> GPHMATGQDRVVALVDMDCFFVQVEQRQNPHLRNKPCAVVQYKSWKGGGIIAVSYEARAFGVTRSMWADDAKKLCPDLLLAQVRESRGKANLTKYREASVEVMEIMSRFAVIERASIDEAYVDLTSAVQERLQKLQGQPISADLLPSTYIEGLPQGPTTAEETVQKEGMRKQGLFQWLDSLQIDNLTSPDLQLTVGAVIVEEMRAAIERETGFQCSAGISHNKVLAKLACGLNKPNRQTLVSHGSVPQLFSQMPIRKIRSLGGKLGASVIEILGIEYMGELTQFTESQLQSHFGEKNGSWLYAMCRGIEHDPVKPRQLPKTIGCSKNFPGKTALATREQVQWWLLQLAQELEERLTKDRNDNDRVATQLVVSIRVQGDKRLSSLRRCCALTRYDAHKMSHDAFTVIKNMNTSGIQTEWSPPLTMLFLCATKFSAS

We show here that human Polη can efficiently bypass AraC embedded in a DNA template strand by incorporating cognate G as well as noncognate deoxynucleotides (predominantly an A) opposite the lesion. In both AraC-containing ternary complexes, Polη encircles the template–primer with its palm (residues 1–13 and 90–238), fingers (residues 17–87), thumb (residues 241–301) domains as well as the PAD (polymerase associated domain; residues 319–432). The palm domain carries the catalytic residues Asp13, Asp115, and Glu116, while the fingers domain lies above the templating AraC base. The thumb and the PAD grasp the template–primer DNA duplex at opposite sides, from the minor and major groove surfaces, respectively.

We crystalized the human Polη catalytic core (residues 1 to 432) with a template-primer 12/8-mer (5′–CAT(AraC)ACAGTGCT–3′/5′–AGCACTGT–3′) and non-reactive dGTP analog dGMPNPP. We refined this cognate ternary complex structure with the G opposite the AraC template residue to 2.4 Å resolution and to Rfree of 21.4% and Rwork of 17.7%. The AraC base pairs with the G base of incoming dGMPNPP with the expectant Watson-Crick (W-C) geometry. However, the C1′- C1′ distance across the base pair is ~10.71 Ả, as compared to 10.5 Ả for an ideal W-C base pair. Also, the AraC base is tilted by ~30°, which negatively impacts its stacking with the adjacent bases on the template strand. The AraC sugar assumes the C1′-exo conformation rather than the C2′-endo conformation observed in Polη structures with unmodified DNA. C1′-exo is one of the preferred sugar conformations for arabinonucleosides, and it appears to be further stabilized in the Polη active by a hydrogen bond between the “extra” 2′-OH on the AraC sugar and the main chain amide of Asn324 of the polymerase. Also, in contrast to the unmodified structures, the side chain of Gln38 forms a hydrogen bond with the O2 atom of the AraC base instead of the O4′ atom the sugar, and Arg61 (unique to Polη) adopts a single rotameric conformation to stabilize the binding of the incoming nucleotide rather than multiple conformations. Importantly, the 3′-OH of the primer terminus is at the reaction-ready distance of 3.41 Ả from the α-P atom of dGMPNPP. Thus, despite local adjustments in how AraC is accommodated in the Polη active site, the polymerase is well poised for the incorporation of G opposite template AraC.> MGFDFNIMVVGQSGLGKSTLVNTLFKSQVSRKASSWNREEKIPKTVEIKAIGHVIEEGGVKMKLTVIDTPGFGDQINNENCWEPIEKYINEQYEKFLKEEVN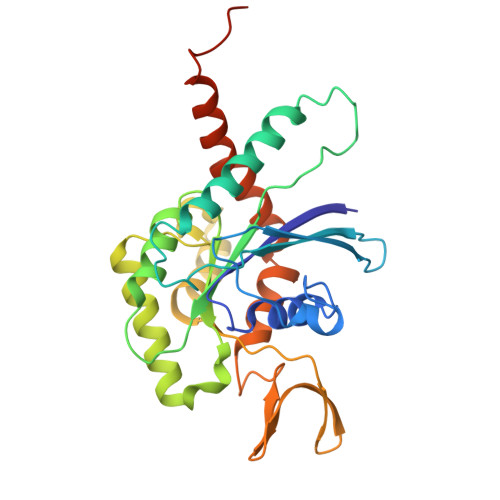IARKKRIPDTRVHCCLYFISPTGHSLRPLDLEFMKHLSKVVNIIPVIAKADTMTLEEKSEFKQRVRKELEVNGIEFYPQKEFDEDLEDKTENDKIRQESMPFAVVGSDKEYQVNGKRVLGRKYPWGIIEVENLNHCEFALLRDFVIRTHLQDLKEVTHNIHYETYRAKRLNDNGGLPPVSVDTEESHDSNP>[4x]HHHHHHSSGLVPRGSHMLLTADTVLTGTELLRPGWLEIASDRVVAVGAGAPPAQADRNLGAATVVPGFVDTHLHGGGGGNFSAATDDETARAV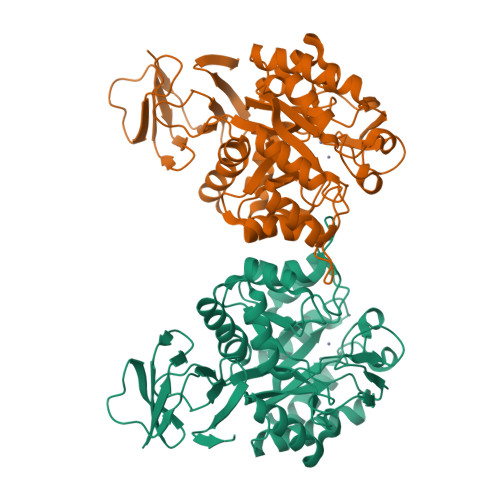ALHRAHGSTTLVASLVTAGPEDLLRQVSGLARQVRAGLIDGIHLEGPWLSTLRCGAHQPVLMRDPDPGEIGRVLDAGEGTVRMVTIAPERDGALAAIAQLVNAGVVAAVGHTEATYDQTRAAIDAGATVGTHLFNAMRPIDRREPGPAVALTEDSRVTVEMIVDGVHVAPAIYRHITQTVGPERLSLITDAMAATGMSDGVYRLGPLDIDVVAGVARVAGTDTIAGSTATMEQVFRLAVAHCGLPRDDALSLAVRQACVNPARALGLPAAGLAAGARADLVVLDHDLAVTAVMRAGEWVVTPGAAHTV>[4x]MASHDKQFSLFLHKASAHGWKVAFVLEELSLSYEIVLV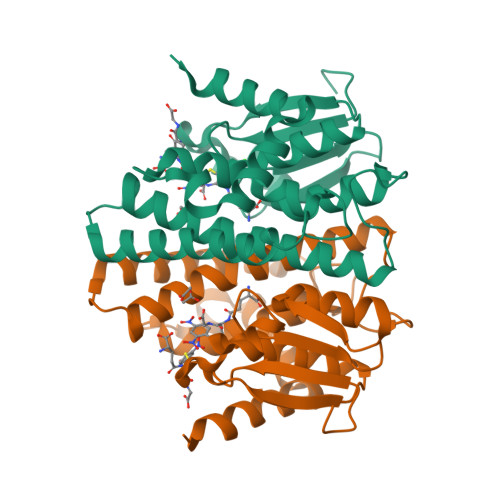DVAKNEQKSPEFMKLNPNGRTPALIDHGNSDFVIWESNAMVQYVADKYDTERKISMAPGTDDFYIQLQWQYFQGTGQGPYFGQLVWFTLYHEEKIPSAVTRYKEEALRVFSVLERVLSNQEWLVGGKMTIADISFVSWNDMIVHFLDNFDFEKEFPATAAWHYKMLKRPTIKRPWDERRKLMSRQ> VRITQGTFSFLPDLTDEQIKKQIDYMISKKLAIGIEYTNDIHPRNAYWEIWGLPLFDVTDPAAVLFEINACRKARSNFYIKVVGFSSVRGIESTIISFIVNRPKHEPGFNLMRQEDKSRSIKYTIHSYESYK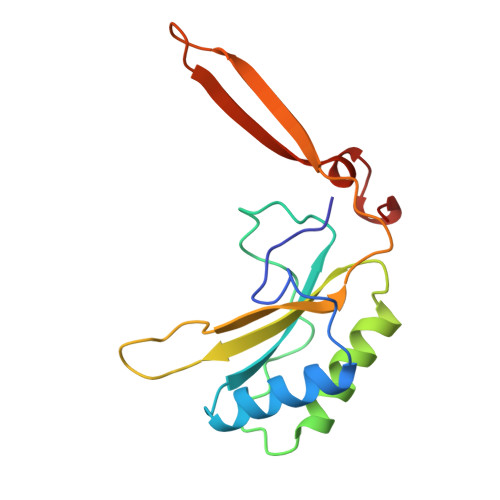PEDERY>ADPHFLQQPEDMVVLLGEEARLPCAL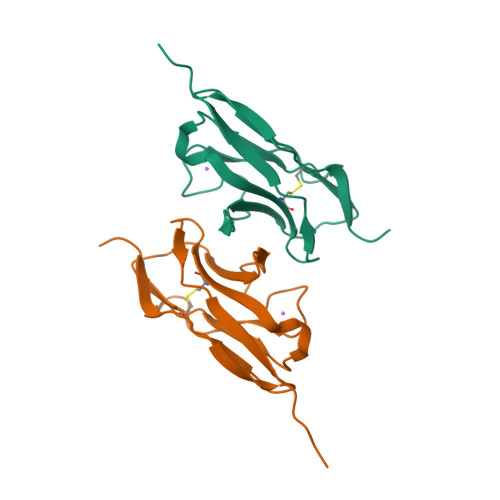GAYRGLVQWTKDGLALGGERDLPGWSRYWISGNSASGQHDLHIKPVELEDEASYECQASQAGLRSRPAQLHVMVPHHHHHH[2x]ADP-ribosyl-acceptor hydrolase 3 (ARH3) cleaves PAR and mono(ADP-ribosyl)ation at serine following DNA damage. In contrast, ARH3 has a unique ARH fold and a di-Mg2+-containing catalytic center and can efficiently reverse not only PARylation but also mono(ADP-ribosyl)ation (MARylation) at serine; ARH3 can also cleave O-acetyl-ADPR and α-NAD+ in a Mg2+-dependent manner releasing free ADPR. While coordination of two magnesium ions (MgA and MgB) significantly enhances its catalytic efficiency, calcium binding suppresses its function. In the active site of ARH3, acidic residues, including Asp77, Asp78, Asp314, and Asp316, maintain the integrity of the bimetallic center and render the ideal alignment of the substrate for catalysis.

To gain further structural basis for different alterations in enzymatic activity in D77A and D314A mutants and to better understand the roles of each Mg2+ ion in ARH3, we determined the high-resolution crystal structures of ARH3D77A and ARH3D314A bound to ADPR and Mg2+ at a resolution of 1.85 and 1.80 Å, respectively. In WT ARH3, Asp77 not only interacts with 2″-OH of the terminal ribose but also coordinates MgA. Thus, Asp77 appears to be important for the maintenance of integrity of MgA and the optimal orientation of the terminal ribose for catalysis. Structural analysis of ARH3D77A reveals that MgA is missing. This lack of MgA causes a large-scale rearrangement in the active site. First, the terminal ribose is rotated ∼37° using MgB as a pivot. Because of this rotation, which is an even greater degree of rotation than that found in the Ca2+-bound form of ARH3, the 2″-OH group replaces the metal-bridging μ-aqua ligand and directly interacts with MgB. In this conformation, the 2″-OH group makes additional hydrogen bonds with side chains of Asp78 and Asp316, and the 1″-OH group makes a new hydrogen bond with the main carbonyl chain of Gly115. Consistently, ARH3D77A shows a 23-fold increase in ADPR-binding affinity, compared with ARH3WT. As a result, the 1″-OH group is displaced ∼2.4 Å toward Ala77.

>[4x]GPHMAAAAMAAAAGGGAGAARSLSRFRGCLAGALLGDCVGSFYEAHDTVDLTSVLRHVQSLEPDPGTPGSERTEALYYTADTAMARALVQSLLAKEAFDEVDMAHRFAQEYKKDPDRGYGAGVVTVFKKLLNPKCRDVFEPARAQFNGKGSYGNGGAMRVAGISLAYSSVQDVQKFARLSAQLTHASSLGYNGAILQALAVHLALQGESSSEHFLKQLLGHMEDLEGDAQSVLDARELGMEERPYSSRLKKIGELLDQASVTREEVVSELGNGIAAFESVPTAIYCFLRCMEPDPEIPSAFNSLQRTLIYSISLGGDTDTIATMAGAIAGAYYGMDQVPESWQQSCEGYEETDILAQSLHRVFQKS>[2x]MMEKLKEIEKVTKAIKEKILNHYGYIRVITHHDTDGLSSGGIL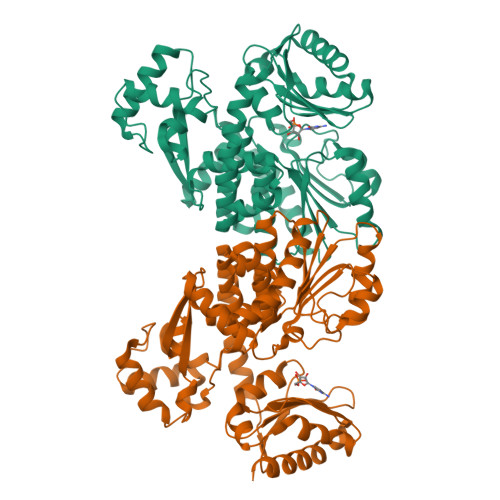AKMLMRTNKLFHLTVVEHLSKEVIEKLAKENEVNKPLFIFADMGSGQIEEIIKHNFNAIILDHHPPVIKDSFINENIIQLNPHIFGVDGSREITASGVCYLVAREFGYYDLSVLAIVGIIGDMQYNPLLGLNKFIVNEAREYRYVKIMNDIVYNIYDVEIYKAIAYCTKPYIPDLASEGKAFKFLKDIGIDPNKKQLDDTDKKKLLSAIIFKYPKIENLLIDRYLIEHKVRDAFLLSEMLNAVGRNGLFAVGIGICLEDDECIKIGNQILWEYKKNLINELKSVKLKKLNNIYYFEGKKGMIGIIASILVDDKPVIGYHIEGDIAKFSARGNRDLVNRGLNLSVAMAVAKEFGGNGGGHDVASGAVVSKDKVQEFLKRVDEIIGEQLRR>GSHMIILKLGGSVITRKDSEEPAIDRDNLERIASEIGNASPSSLMIVHGAGSFGHPFAGEYRIGSEIENEEDLRRRRFGFALTQNWVKKLNSHVCDALLAEGIPAVSMQPSAFIRAHAGRISHADISLIRSYLEEGMVPVVYGDVVLDSDRRLKFSVISGDQLINHFSLRLMPERVILGTDVDGVYTRNPKKHPDARLLDVI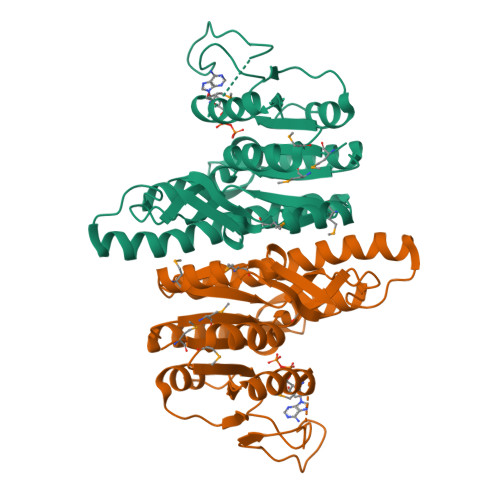GSLDDLESLDGTLNTDVTGGMVGKIRELLLLAEKGVESEIINAAVPGNIERALLGEEVRGTRITGKH[2x]> MHHHHHHAMAIHSGPASTSFGVNVFKQMATEQSGNLAASPFSITILLAMLQQGAAGNTLDEITRALQMTPEKSAEIFKKVNEEIQKRNSRNILKTANNV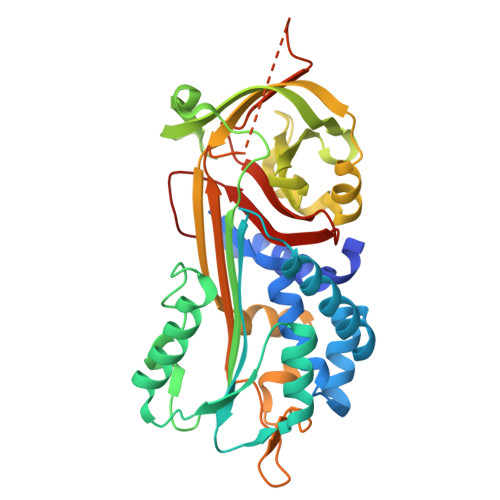FLSENFNLNPQFKRIAVNNFDSDLTPTYFGKPALAAQNINSWIASKTNDKIDKLVSPDDLSGNTQMVMVNAVYFKGLWEIPFREQATQKRNFTLNGGEKKVASFMQTRRYFKAGTHKPAMAKVVVLPFEYNEYSLIVVLPLKSSNVDALLSSLSMEDVASFLDLPPKDVALELPKFSIKADINLEPVLNKMGVSSIFTQQAELYNLGSHGSLSPQVSSALHSAVLTIDERGGSAAAATSFAAVALSYDEPSLYFRANKPFLAILWDNRSSIPLFMARIMDPTLEHARAAEV> FQGAMSSSIDISKINSWNKEFQSDLTHQLATTVLKNYNADDALLNKTRLQKQDNRVFNTVVSTDSTPVTNQKSSGRCWLFAATNQLRLNVLSELNLKEF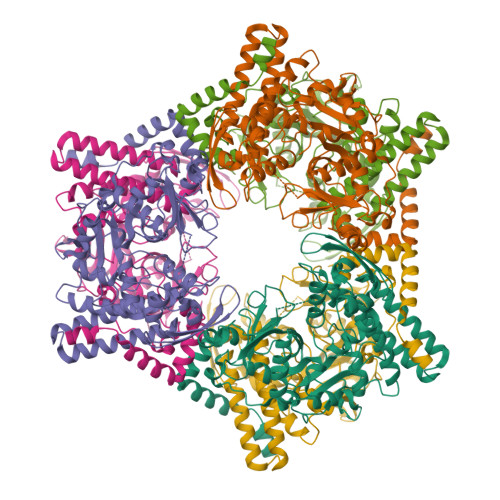ELSQAYLFFYDKLEKANYFLDQIVSSADQDIDSRLVQYLLAAPTEDGGQYSMFLNLVKKYGLIPKDLYGDLPYSTTASRKWNSLLTTKLREFAETLRTALKERSADDSIIVTLREQMQREIFRLMSLFMDIPPVQPNEQFTWEYVDKDKKIHTIKSTPLEFASKYAKLDPSTPVSLINDPRHPYGKLIKIDRLGNVLGGDAVIYLNVDNETLSKLVVKRLQNNKAVFFGSHTPKFMDKKTGVMDIELWNYPAIGYNLPQQKASRIRYHESLMTAAMLITGCHVDETSKLPLRYRVENSWGKDSGKDGLYVMTQKYFEEYCFQIVVDINELPKELASKFTSGKEEPIVLPIWDPMGALA>MSKTFAEIAEAFLEPEAVRIAKEAVEEYGDHERKIIQIGIHFQVCCMFCDEYLSTNGSDRFVLIEGRKRGTAVSLQNELCKSYDLEPLPFLCDIFDREEKQFVEIGITRKADDSYFQSKFGKLGNSCKIFVFSYDGRLDKNCEGPMEEQKLRIFSFLATAADFLRKENMFNEIFLPDNEETIIEMKKGKTFLELRDESVPLPFQTYEQMKDYCEKFKGNPRELASKVSQMQSNIKLPIKHYEQNKFRQIRLPKGPMAPYTHKFLMEEAWMFTKISDPERSRAGEILIDFFKKGNLSAIRPKDKPLQGKYPIHYKNLWNQIKAAIADRTMVINENDHSEFLGGIGRASKKIPEISLTQDVITTEGLKQSENKLPEPRSFPRWFNAEWMWAIKDSDLTGWVPMAEYPPADNELEDYAEHLNKTMEGVLQGTNCAREMGKCILTVGALMTECRLFPGKIKVVPIYARSKERKSMQEGLPVPSEMDCLFGICVKSKSHLNKDDGMYTIITFEFSIREPNLEKHQKYTVFEAGHTTVRMKKGESVIGREVPLYLYCRTTALSKIKNDWLSKARRCFITTMDTVETICLRESAKAEENLVEKTLNEKQMWIGKKNGELIAQPLREALRVQLVQQFYFCIYNDSQLEGFCNEQKKILMALEGDKKNKSSFGFNPEGLLEKIEECLINNPMCLFMAQRLNELVIEASKRGAKFFKTD[2x];>[2x]MEINPYLMFLNNDVTSLISTTYPYTGPPPMSHGSSTKYTLETIKRTYDYSRTSVEKTSKVFNIPRRKFCNCLEDKDELVKPTGNVDISSLLGLAEMMEKRMGEGFFKHCVMEAETEILKMHFSRLTEGRQTYDWTSERNMPAATALQLTVDAIKETEGPFKGTTMLEYCNKMIEMLDWKEIKFKKVKTVVRREKDKRSGKEIKTKVPVMGIDSIKHDEFLIRALTINTMAKDGERGKLQRRAIATPGMIVRPFSKIVETVAQKICEKLKESGLPVGGNEKKAKLKTTVTSLNARMNSDQFAVNITGDNSKWNECQQPEAYLALLAYITKDSSDLMKDLCSVAPVLFCNKFVKLGQGIRLSNKRKTKEVIIKAEKMGKYKNLMREEYKNLFEPLEKYIQKDVCFLPGGMLMGMFNMLSTVLGVSTLCYMDEELKAKGCFWTGLQSSDDFVLFAVASNWSNIHWTIRRFNAVCKLIGINMSLEKSYGSLPELFEFTSMFFDGEFVSNLAMELPAFTTAGVNEGVDFTAAMSIIKTNMINNSLSPSTALMALRICLQEFRATYRVHPWDSRVKGGRMKIINEFIKTIENKDGLLIADGGKLMNNISTLHIPEEVLKFEKMDEQYRNRVFNPKNPFTNFDKTIDIFRAHGPIRVEENEAVVSTHSFRTRANRTLLNTDMRAMMAEEKRYQMVCDMFKSVFESADINPPIGAMSIGEAIEEKLLERAKMKRDIGAIEDSEYEEIKDIIRDAKKARLESR;>[2x]MSLLLTIAKEYKRLCQDAKAAQMMTVGTVSNYTTFKKWTTSRKEKNPSLRMRWAMSSKFPIIANKRMLEEAQIPKEHNNVALWEDTEDVSKRDHVLASASCINYWNFCGPCVNNSEVIKEVYKSRFGRLERRKEIMWKELRFTLVDRQRRRVDTQPVEQRLRTGEIKDLQMWTLFEDEAPLASKFILDNYGLVKEMRSKFANKPLNKEVVAHMLEKQFNPESRFLPVFGAIRPERMELIHALGGETWIQEANTAGISNVDQRKNDIRAVCRKVCLAANASIMNAKSKLVEYIKSTSMRIGETERKLEELILETDDVSPEVTLCKSALGGQLGKTLSFGPMLLKKISGSGVKVKDTVYIQGVRAVQFEYWSEQEEFYGEYKSATALFSRKERSLEWITIGGGINEDRKRLLAMCMIFCRDGDYFKDAPATITMADLSTKLGREIPYQYVMMNWIQKSEDNLEALLYSRGIVETNPGKMGSSMGIDGSKRAIKSLRAVTIQSGKIDMPESKEKIHLELSDNLEAFDSSGRIVATILDLPSDKKVTFQDVSFQHPDLAVLRDEKTAITKGYEALI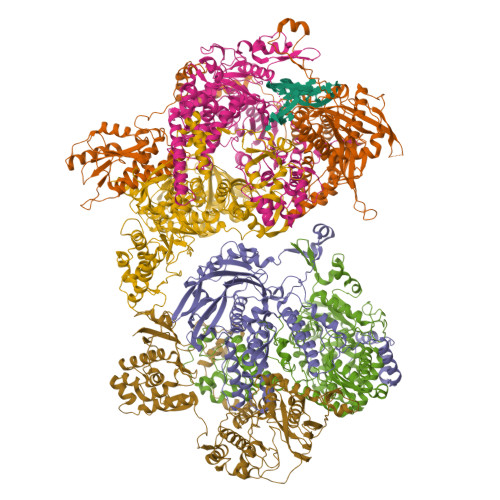KRLGTGDNDIPSLIAKKDYLSLYNLPEVKLMAPLIRPNRKGVYSRVARKLVSTQVTTGHYSLHELIKVLPFTYFAPKQGMFEGRLFFSNDSFVEPGVNNNVFSWSKADSSKIYCHGIAIRVPLVVGDEHMDTSLALLEGFSVCENDPRAPMVTRQDLIDVGFGQKVRLFVGQGSVRTFKRTASQRAASSDVNKNVKKIKMSN1-(1-methylethyl)-1H-benzimidazole-2-sulfonic 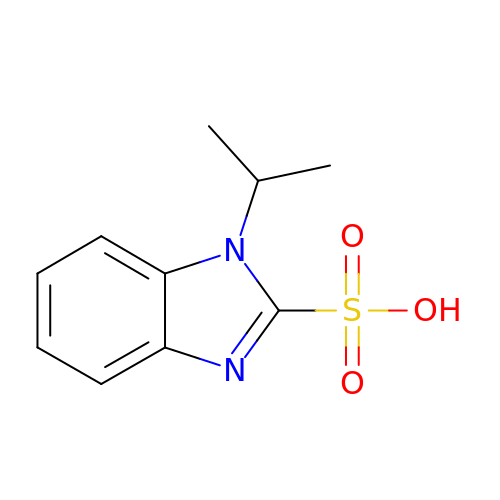acid | C10 H12 N2 O3 S | ZSZNPVDVEUJQJS-UHFFFAOYSA-N> SMVEATGNNCPPHIESFSDVEMGEIIMGNIELTRYTRPTPVQKHAIPIIKEKRDLMACAQTGSGKTAAFLLPILSQIYSDGPGEALRAMKENGRYGRR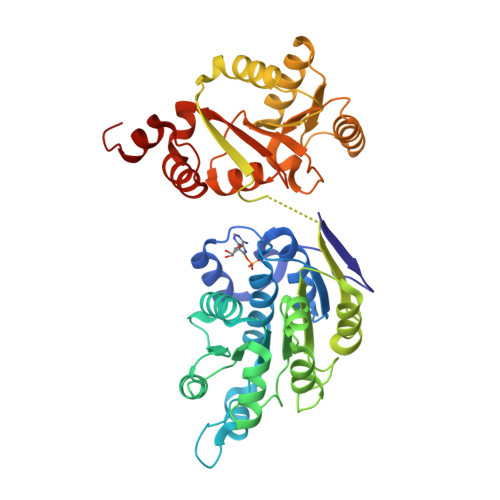KQYPISLVLAPTRELAVQIYEEARKFSYRSRVRPCVVYGGADIGQQIRDLERGCHLLVATPGRLVDMMERGKIGLDFCKYLVLDEADRMLDMGFEPQIRRIVEQDTMPPKGVRHTMMFSATFPKEIQMLARDFLDEYIFLAVGRVGSTSENITQKVVWVEESDKRSFLLDLLNATGKDSLTLVFVETKKGADSLEDFLYHEGYACTSIHGDRSQRDREEALHQFRSGKSPILVATAVAARGLDISNVKHVINFDLPSDIEEYVHRIGRTGRVGNLGLATSFFNERNINITKDLLDLLVEAKQEVPSWLENMAYEHHYKG> MELADVGAAASSQGVHDQVLPTPNASSRVIVHVDLDCFYAQVEMISNPELKDKPLGVQQKYLVVTCNYEARKLGVKKLMNVRDAKEKCPQLVLVNGEDLTRYREMSYKVTELLEEFSPVVERLGFDENFVDLTEMVEKRLQQLQSDELSAVTVSGHVYNNQSINLLDVLHIRLLVGSQIAAEMREAMYNQLGLTGCAGVASNKLLAKLVSGVFKPNQQTVLLPESCQHLIHSLNHIKEIPGIGYKTAKCLEALGINSVRDLQTFSPKILEKELGISVAQRIQKLSFGEDNSPVILSGPPQSFSEEDSFKKCSSEVEAKNKIEELLASLLNRVCQDGRKPHTVRLIIRRYSSEKHYGRESRQCPIPSHVIQKLGTGNYDVMTPMVDILMKLFRNMVNVKMPFHLTLLSVCFCNLKALNTAK

Humans have four Y-family polymerases – Polι, Polη, Polκ, and Rev1 – each with a unique DNA damage bypass and fidelity profile. Amongst these, Polι stands out in that it does not rely on W-C base pairing between the template base and incoming nucleotide for catalysis. Instead, the active site cleft of Polι is much narrower than in other DNA polymerases, favoring Hoogsteen base pairing. As such, Polι would appear to be well suited to bypass 1-MeA, which has an altered W-C edge but an intact Hoogsteen edge.

The Polι1-MeA.dTTP ternary complex (Rfree of 24.9%, Rcryst of 20.5%) was refined to 2.6 Å resolution and contains Polι residues 26–350, 356–371, 378–397 and 403–414, DNA nucleotides 3–11, incoming dTTP, 1 Mg2+ ion, 1 Cl− ion, and 87 water molecules. Clear electron density was visible for both the template 1-MeA and the incoming dTTP in initial Fo-Fc and simulated annealing Fo-Fc omit maps for Polι1-MeA.dTTP. Template 1-MeA is similarly observed in the syn conformation, presenting its Hoogsteen edge for hydrogen bonding with dTTP which remains in the anti conformation. The 1-MeA and dTTP bases are almost coplanar and two putative hydrogen bonds are established between the N6 and N7 atoms of 1-MeA with the O4 and N3 atoms of T (2.8 Å and 3.2 Å respectively). The 1-MeA.T base pair is isomorphic with the A.T and εdA.T base pairs in the structures of PolιdA.dTTP and PolιεdA.dTTP, respectively. Incoming dTTP is anchored at one end of the dNTP binding cavity by hydrogen bonding interactions between its γ-phosphate and the side chains of Tyr68 and Arg71 from the fingers domain and Lys214 from the palm domain. At the other end, Hoogsteen base pairing with 1-MeA secures the base of dTTP in the binding pocket. A single Mg2+ ion (metal B) is coordinated by the triphosphate moiety of dTTP, as well as the active site residues Asp34 and Asp126. In Polι1-MeA.dTTP (and other ternary structures with purine templates), the side chain of Asp126 undergoes an ~30° rotation to establish new interactions with the backbone carbonyl of Leu35, the metal ion at site B, and with the α-phosphate of incoming dNTP. Overall, Polι1-MeA.dTTP is well poised for catalysis with a 3′-OH modeled at the primer terminus located ~3.1 Å from the dTTP α-phosphate and aligned more or less linearly with respect to the scissile Pα-O3′ bond (~162°).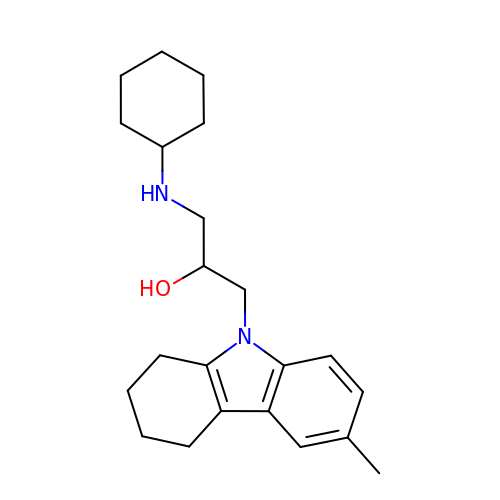1-(CYCLOHEXYLAMINO)-3-(6-METHYL-3,4-DIHYDRO-1H-CARBAZOL-9(2H)-YL)PROPAN-2-OL | C22 H32 N2 O | AXYFCRIRLKSCRR-SFHVURJKSA-N We have been interested in a D-aminoacyl-tRNA deacylase (DTD) fold that is present across the domains of life in two different functional contexts: as an N-terminal editing domain (NTD) of archaeal ThrRS, which specifically removes non-cognate L-serine mischarged on tRNAThr, and as a freestanding ‘chiral proofreading' enzyme, which removes D-amino acids from tRNAs in bacteria and eukaryotes. Both share a striking structural and mechanistic similarity highlighting a common ancestry. Here we show, with the help of structural, biochemical and biophysical studies from three distant organisms, that the substrate specificity in this domain is determined by a differential remodelling of the catalytic centre at the RNA–protein interface rather than just the presence or absence of catalytic water as previously proposed. While demonstrating that the tRNA provides the catalytic group, we show that the side chains within the recognition site are dispensable for the proofreading function, suggesting a primordial mode of protein- or peptide scaffold-based enzymatic activity evolved alongside that of RNA.

To understand this intriguing mechanism of cognate substrate rejection in NTD, we have solved high-resolution crystal structures of ApNTD, as well as NTD from Methanococcus jannaschii (MjNTD) in complex with non-cognate and cognate substrate analogues L-seryl-3′-aminoadenosine (L-Ser3AA) and L-threonyl-3′-aminoadenosine (L-Thr3AA), respectively. The co-crystal structures of ApNTD were solved in P41212 space group with only one monomer in the asymmetric unit, as the biological dimer axis coincided with the crystallographic twofold axis. L-Ser3AA tightly binds in the active-site pocket in such a way that a conserved hydrogen bond with the main-chain N atom of Lys121 (residue number corresponding to PabNTD) fixes the β-OH group of the substrate in all three NTDs. The carbonyl oxygen of the substrate has a water-mediated interaction with His83 in PabNTD, while the same atom interacts directly with the corresponding His77 in ApNTD and His84 in MjNTD. However, in ApNTD, it has only a water-mediated interaction with the corresponding Glu129, whereas in the case of MjNTD, this group is directly recognized by both Glu135 and His84. In ApNTD, on the other hand, the extra space in the vicinity of Wat1 allows a second ApNTD-specific water Wat5 to be accommodated. Therefore, to ensure that the loosening of interactions observed in ApNTD is significant, we solved multiple high-resolution crystal structures of this enzyme with L-Ser3AA and L-Thr3AA to obtain random snapshots of the substrate analogue in the active site. The average interaction distances of the ligand atoms coming from four L-Ser3AA-bound structures and four L-Thr3AA-bound structures clearly demonstrate a general loosening of the aminoacyl moiety upon L-Thr3AA binding.

> MRLLYLHADRFEYKTVKPALKNPPDPPGEASFGEALVVFTTVEDGDGPQTVMYAASDIASHSSRLKVTTVILYPYAHLSSRLAKPMAAHKRLIELEGALRTKFPGHVHRAPFGWYKSFSIACKGHPLAELSRSFTE>[2x]DNNVLLTGDVIHTDNQLSYESAAFVMQGDCNLVLYNEAGGFQSNTHGRGVDCTLRLNNRGQL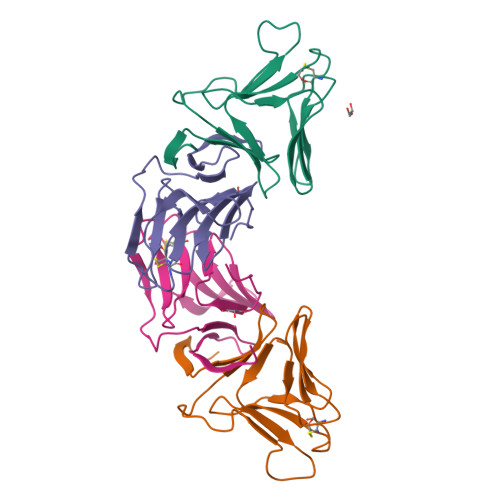EIHSANSNTPVWVYPRSVNTVRGNYAATLGPDQHVTIYGPAIWSTPAAA;>NIPRVRNVLFSSQVMYDNAQLATRDYSLVMRDDCNLVLTKGSKTNIVWESGTSGRGQHCFMRLGHSGELDITDDRLNTVFVSNTVGQEGDYVLILQINGQAVVYGPAVWSTAA[2x]QPRTs have been shown to exist as dimers or hexamers2223242526272829. HsQPRT is regulated by the interaction between two dimeric subunits. which can adopt open and closed states.

complex with QA or NAMN as a reactant or product. the product and form a hexamer in the HsQPRT-open structure. product complex to have a more relaxed hexamer. may provide the driving force to release NAMN.

>[12x]MDAEGLALLLPPVTLAALVDSWLREDCPGLNYAALVSGAGPSQAALWAKSPGVLAGQPFFDAIFTQLNCQVSWFLPEGSKLVPVARVAEVRGPAHCLLLGERVALNTLARCSGIASAAAAAVEAARGAGWTGHVAGTRKTTPGFRLVEKYGLLVGGAASHRYDLGGLVMVKDNHVVAAGGVEKAVRAARQAADFALKVEVECSSLQEAVQAAEAGADLVLLDNFKPEELHPTATVLKAQFPSVAVEASGGITLDNLPQFCGPHIDVISMGMLTQAAPALDFSLKLFAKEVAPVPKIHLEHHHHHH> RTPSDKPVAHVVANPEAEGQLQWLSRRANALLANGVELTDNQLIVPSDGLYLIYSQVLFKGQGCPSTHVLLTHTISRFAVSYQTKVNLLSAIKSPCQRETPEGTEAKPWYEPIYLGGVFQLEKGDRL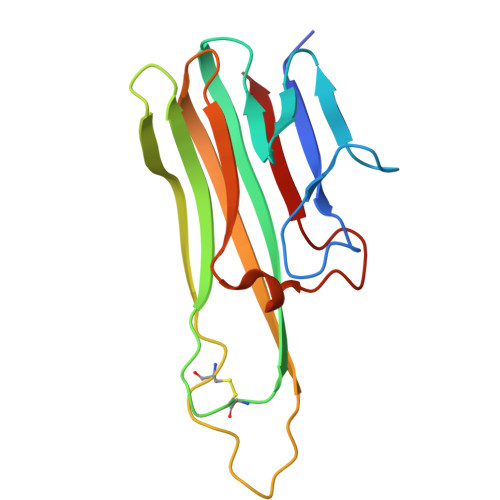SAEINLPNYLDFAESGQVYFGIIAL> MTVLHWATISPFLLAILIPFLYKYARRIHTGWFVLALPLVLFIYFIRYLSVTSTGGVVEHTIPWVPSLGINFTVFVDGLSLLFALLITGIGTLVILYSIFYLSKKTESLNNFYVYLLMFMGAMLGVVLSDNLIVLYVFWELTSLASSLLISYWFHREKSTYGAQKSMLITVFGGFAMLGGFSLLYVMTGTFSIRGIIENVDLVTSSELFLPAMILVLLGAFTKSAQFPFHIWLPDAMEAPTPVSAYLHSATMVKAGIYLVARLTPVFAGSAEWFWLLTGFGVVTLLWGSTSAVRQKDLKGILAFSTVSQLGLIMTLLGLGSAA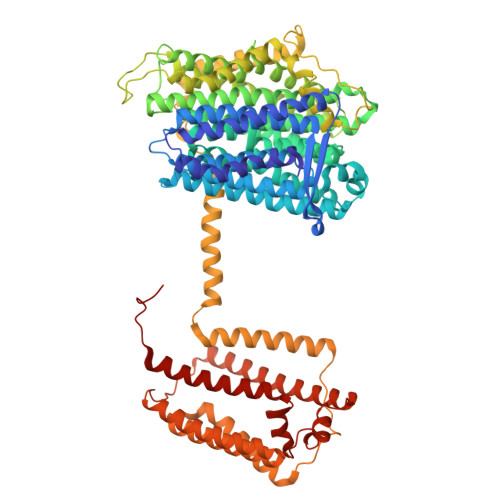IYFGDSVDPAFYSFAIMAAIFHLINHATFKGSLFMTAGIIDHETGTRDIRKLGGLMAIMPVTFTVSLIGLASMAGLPPFNGFLSKEMFFTALLRATEMNTFNMETFGIIIVVLAWIASVFTFLYCLIMFFKTFTGKFKPENYDVKVHEAPIGMLISPVILGSLVIVFGFFPNILAYTIIEPAMQAILPTLLADGEVFYVNIYMWHGFNAELFMTMGVVAAGIILFLMMKNWAKTAFYMKERDPLNWFYDNSLSGVITGSQAVTRIQMTGLLRDYFAYMTTFMILLLGYTMFRYDAFTIDTTNVTGIAPYIWVITLVFIAATLSIPFINKRITAVVVVGVIGFLLALLFVVFRAPDLALTQLLVETVTVLLLMLAFYHLPELRKEEFKPRFNIVNLIISIGVGFLVTAIALSSLALGNEAGIEPISQFFVENSKELAGGYNMVNVILVDFRGLDTLLEVLVLGIAALGVIALIKLRMTGREDV> MGTGRIHALALFFALALFLLGLRAWQLQVLEYERYALRSQGNYLKTEDIPAPRGKILDRKGRVLAQDRLVVDLVYTGGEVAFKERLLPLLGLEDLPQVTEPTVLKAGVPEALRPTLEELTAGQKNLYLRERIERYYPNPISGPVMGYVLRANAAQVKQGYSPEEEVGQAGLEAALEPYLRGKRGVRAVEVNVRGERLRETVLEEPTPGQDVVLTLDLALQRAAEKALEEALADINAGRRLNGLPEEKQVKGAIVALDPTTGEVLAMASAPSFDPNLFAKRPVPEEAKALLEDKNLPLLNRAVQPYTPGSTFKLATSYALLEEGYVTPATTYRCSPYIVFGGQVR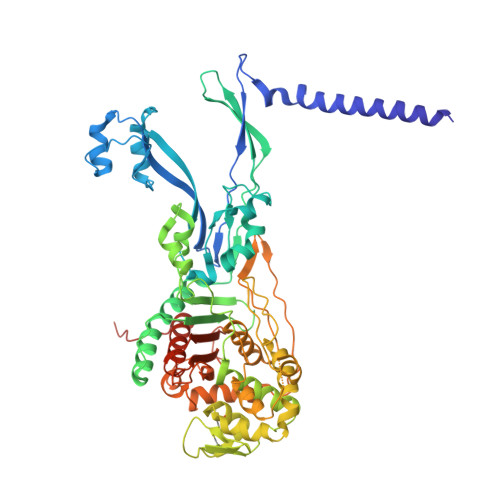RNWASRDMGPMTVREAIAWSCNTWYYQAVAQDPLGFVDRLARRARLLGLGEATGLEVAEKTGLLPTRAWKREALGEPWYPGETLSVAIGQGAVLATPAQIARMLATIATGGNKPALHLVKAIGGVPVQPRWEKVPGRYWKVLQEGLRKTVSEGTARFVLGEFPVPTGGKTGTAETPGKRRGLEHAWYMGYGPTDGSPYPPLVVVAFFENGGEGSRVALPAVRKVMAAYWGIKGSLEVLFQGPEDQVDPRLIDGK>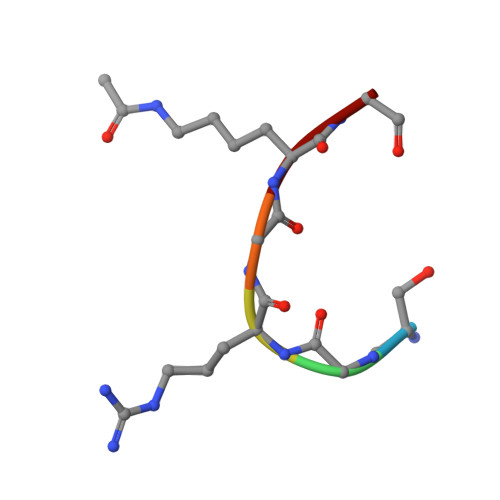 SGRGKG> MQKQILTSQKRNMYILSRCKVLVKNGQVCHLHEDGNVYTVPYANTVFIGLAEGTSITNEAMSMLAANGVIVFWTKGGGYDMFAADIICHLPQADYRPTKYMQNWVRLWLDEEKKLSAAKEILKMRVDSLSTHVHDFGVDVENKRVSSIVNKFDKGVTQATSFESLLGHEGTFVKSLYKEYALEYEIEFKRDHKSADNYNK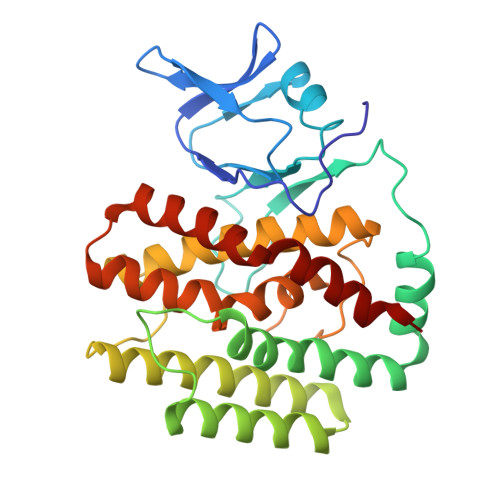FLTLGNYYAYGIARSSLWALGIDNSFPLLHGSTRRGGLVFDVADIIKTSIILPLAFHAADQGMSNTEFKRSCVAYFDKNDILAYLINNIKRLCME> MLPKDKLNPPTPSIYLENKRDAFFPPLHQFCTNPKNPVTVIRG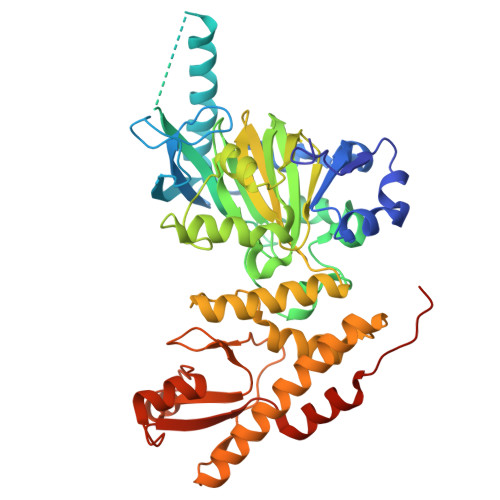LAGALKLDLGLFSTKTLVEANNEHMVEVRTQLLQPADENWDPTGTKKIWRCESNRSHTTIAKYAQYQASSFQESLREENEKRTQHKDHSDNESTSSENSGRRRKGPFKTIKFGTNIDLSDNKKWKLQLHELTKLPAFARVVSAGNLLTHVGHTILGMNTVQLYMKVPGSRTPGHQENNNFCSVNINIGPGDCEWFVVPEDYWGVLNDFCEKNNLNFLMSSWWPNLEDLYEANVPVYRFIQRPGDLVWINAGTVHWVQAVGWCNNIAWNVGPLTACQYKLAVERYEWNKLKSVKSPVPMVHLSWNMARNIKVSDPKLFEMIKYCLLKILKQYQTLREALVAAGKEVIWHGRTNDEPAHYCSICEVEVFNLLFVTNESNTQKTYIVHCHDCARKTSKSLENFVVLEQYKMEDLIEVYDQFTLALSLSSSSAENLYFQ L-ribulose | C5 H10 O5 | 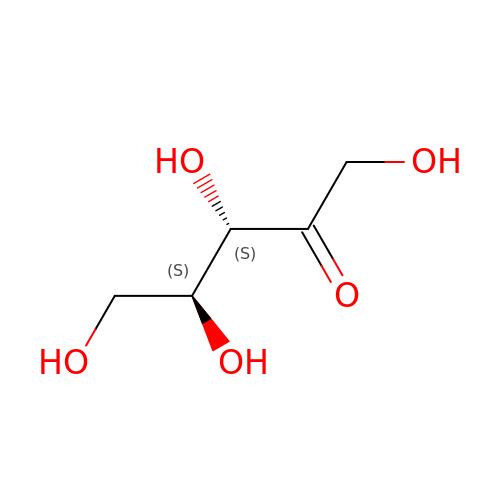ZAQJHHRNXZUBTE-UCORVYFPSA-N>MHHHHHHNLALNKATATSSIET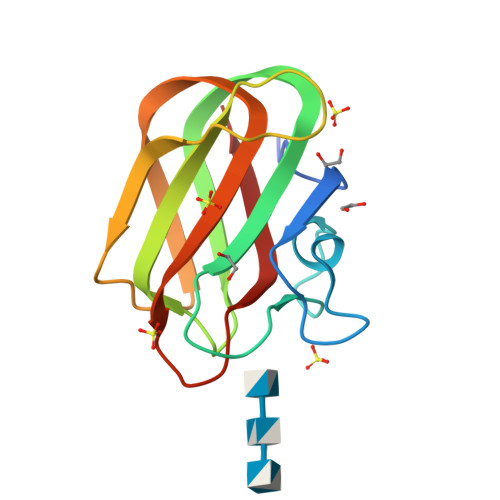AGHEGDKAVDGNAATRWASAYGASPQWIYINLGSTQSISRVKLNWEDAYATAYSIQVSNDSGSTPTNWTTVYSTTTGDGAIDDITFAATNAKFVRVYATTRATAYGYSLWEFEVYG[2x]>IIGGHEVTPHSRPYMASVRFGGQHHCGGFLLRARWVVSAAHCFSHRDLRTGLVVLGAHVLSTAEPTQQVFGIDALTTHPDYHPMTHANDICLLRLNGSAVLGPAVGLLRLPGRRARPPTAGTRCRVAGWGFVSDFEEL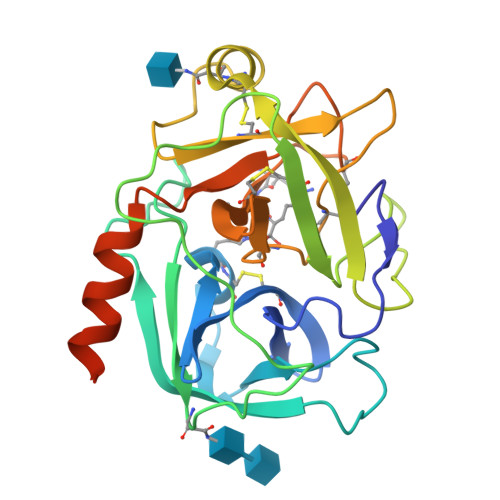PPGLMEAKVRVLDPDVCNSSWKGHLTLTMLCTRSGDSHRRGFCSADSGGPLVCRNRAHGLVSFSGLWCGDPKTPDVYTQVSAFVAWIWDVVRRSSPQPGPLPGTTRPPGEAA[2x]>[2x]PHPICEVSKVASHLEVNCDKRNLTALPPDLPKDTTILHLSENLLYTFSLATLMPYTRLTQLNLDRCELT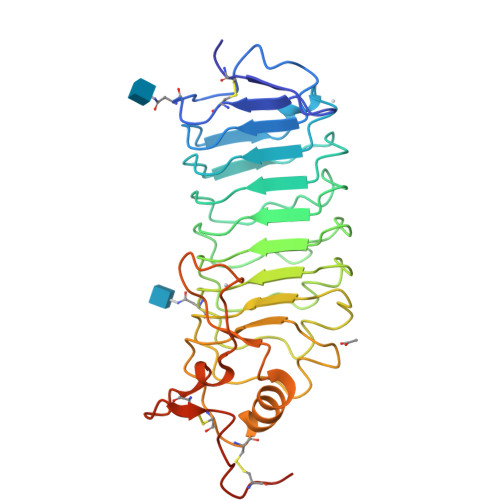KLQVDGTLPVLGTLDLSHNQLQSLPLLGQTLPALTVLDVSFNRLTSLPLGALRGLGELQELYLKGNELKTLPPGLLTPTPKLEKLSLANNNLTELPAGLLNGLENLDTLLLQENSLYTIPKGFFGSHLLPFAFLHGNPWLCNCEILYFRRWLQDNAENVYVWKQGVDVKAMTSNVASVQCDNSDKFPVYKYPGKGCPTLGDEGDTDLYDYYP>[3x]IDYKFWYTQPVPKINDEFNESVNEPFISDNKVEDVRKDEYKLPPGYSWYVCDVKDEKDRSEIYTLLTDNYVEDDDNIFRFNYSAEFLLWALTSPNYLKTWHIGVKYDASNKLIGFISAIPTDICIHK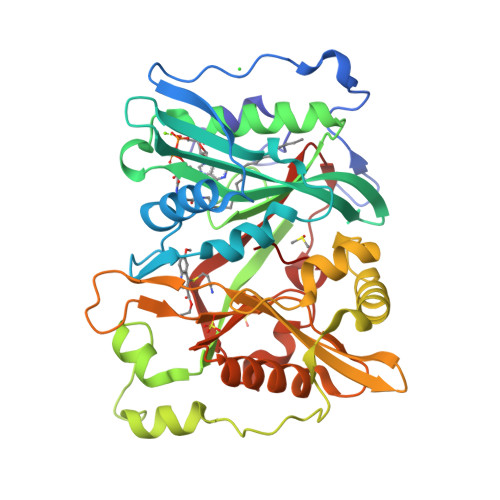RTIKMAEVNFLCVHKTLRSKRLAPVLIKEITRRINLENIWQAIYTAGVYLPKPVSDARYYHRSINVKKLIEIGFSSLNSRLTMSRAIKLYRVEDTLNIKNMRLMKKKDVEGVHKLLGSYLEQFNLYAVFTKEEIAHWFLPIENVIYTYVNEENGKIKDMISFYSLPSQILGNDKYSTLNAAYSFYNVTTTATFKQLMQDAILLAKRNNFDVFNALEVMQNKSVFEDLKFGEGDGSLKYYLYNWKCASFAPAHVGIVLL> MTSITAIFFDLDGTLVDSSIGIHNAFTYTFKELGVPSPDAKTIRGFMGPPLESSFATCLSKDQISEAVQIYRSYYKAKGIYEAQLFPQIIDLLEELSSSYPLYIT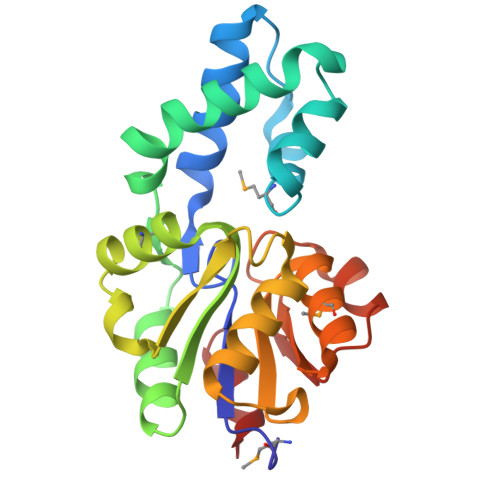TTKDTSTAQDMAKNLEIHHFFDGIYGSSPEAPHKADVIHQALQTHQLAPEQAIIIGDTKFDMLGARETGIQKLAITWGFGEQADLLNYQPDYIAHKPLEVLAYFQ>[2x]NLFVALYDFVASGDNTLSITKGEKLR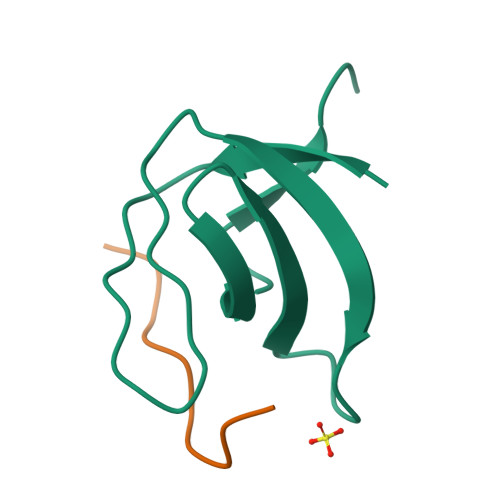VLGYNHNGEWCEAQTKNGQGWVPSAYITPVNS;>[2x]XAPSYSPPPPP>[2x]MTNNNQIGENKEQTIFDHKGNVIKTEDREIQIISKFEEPLIVVLGNVLSDEECDELIELSKSKLARSKVGSSRDVNDIRTSS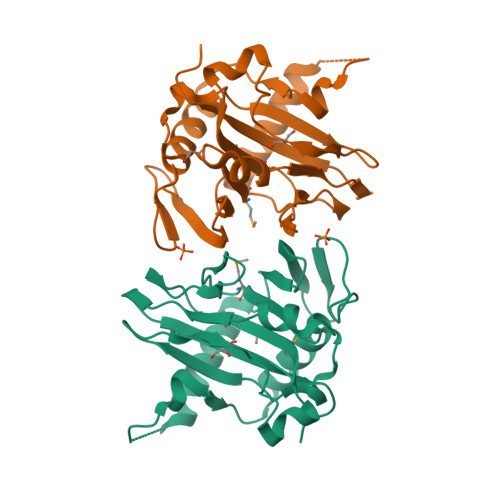GAFLDDNELTAKIEKRISSIMNVPASHGEGLHILNYEVDQQYKAHYDYFAEHSRSAANNRISTLVMYLNDVEEGGETFFPKLNLSVHPRKGMAVYFEYFYQDQSLNELTLHGGAPVTKGEKWIATQWVRRGTYK>MSPILAKNIVYVAQIKGQITSYTYDQFDRYITIAEQDNAEAIIIELDTPGGRADAMMNIVQRIQQSKIPVIIYVYPPGASAASAGTYIALGSHLIAMAPGTSIGACRPILGYSQNGSIIEAPPAITNYFIAYIKSLAQESGRNATIAEEFITKDLSLTPEEALKYGVIEVVARDINELLKKSNGMKTKIPVNGRYVTLNFTNVEVRYLAPSFKDKLISYITDLEHHHHHH[2x];> NVIVLMLPME

The N-terminal region of STOPP PH1510p (residues 16–236, 1510-N) is a thermostable serine protease with a catalytic Ser–Lys dyad (Ser97 and Lys138), and specifically cleaves the C-terminal hydrophobic region of the p-stomatin PH1511p (235VIVL↓MLPM242 in which the arrow indicates the point cleaved). Membrane-bound proteases play several important roles in protein quality control and regulation. In both archaeal and bacterial species, p-stomatin and STOPP (stomatin operon partner protein) genes probably form an operon. The flexible L2 loops of 1510-N cover the peptide, and are involved in the protease activity.

1510-N is a thermostable protease, and the elevated activity was observed with temperatures from 323 to 371 K. Thus, we presume that heat treatment is a good candidate for approaching the second catalytic step of 1510-N. The protein–peptide complex was heated at 353 K for 10 min, and then crystallization trials were performed. Using the heat-treatment complex of 1510-N K138A and 234P10 peptide, crystals were obtained under the condition similar to that of the no heat-treatment complex obtained previously, and the structure was determined. The structure with heat treatment determined here is fitted to the structure with no heat-treatment determined previously, resulting in a low root-mean-square (r.m.s.) difference of 0.15 Å for Cα atoms of the 1510-N dimer, and 0.40 Å for all atoms of the peptide. The result indicates that the structure with heat treatment is almost identical to that with no heat-treatment. The N-terminal half of the peptide (234NVIVL238) shows clear electron densities, whereas the C-terminal half of the peptide (239MLP241) shows weak densities. Almost all the main-chain nitrogen and carboxyl oxygen atoms of 234NVIVL238 are hydrogen-bonded to the protease. The main-chain atoms of 239MLP241 have fewer hydrogen bonds than 234NVIVL238. According to the superposition between the structures with heat-treatment and with no heat-treatment, the 234NVIVL238 peptide is superposed well, whereas the 239MLP241 peptide is slightly deviated. According to the results of hydrogen bonds and superposition, the N-terminal half of the peptide binds to 1510-N more tightly than the C-terminal half of the peptide. The two catalytic Ala138 residues that replaced Lys are located very close together.> SDALKVRWPDFNQEAYVGGTMVRSGQDPYARNKFNQVESDKLRMDRAIPDTRHDQCQRKQWRVDLPATSVVITFHNEARSALLRTVVSVLKKSPPHLIKEIILVDDYSNDPEDGALLGKIEKVRVLRNDRREGL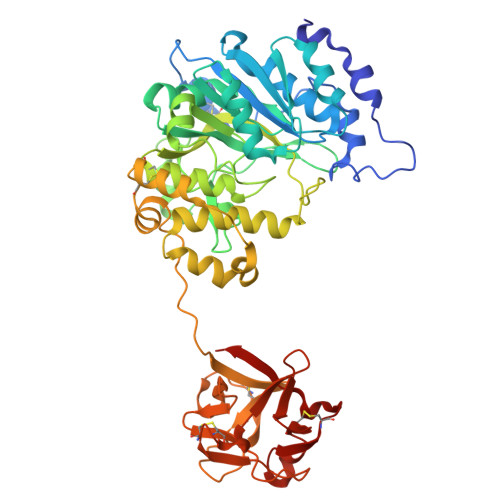MRSRVRGADAAQAKVLTFLDSHCECNEHWLEPLLERVAEDRTRVVSPIIDVINMDNFQYVGASADLKGGFDWNLVFKWDYMTPEQRRSRQGNPVAPIKTPMIAGGLFVMDKFYFEELGKYDMMMDVWGGENLEISFRVWQCGGSLEIIPCSRVGHVFRKQHPYTFPGGSGTVFARNTRRAAEVWMDEYKNFYYAAVPSARNVPYGNIQSRLELRKKLSCKPFKWYLENVYPELRVPDHQDIAFGALQQGTNCLDTLGHFADGVVGVYECHNAGGNQEWALTKEKSVKHMDLCLTVVDRAPGSLIKLQGCRENDSRQKWEQIEGNSKLRHVGSNLCLDSRTAKSGGLSVEVCGPALSQQWKFTLNLQQ> MTAPHDPLDDIQADPWALWLSGRT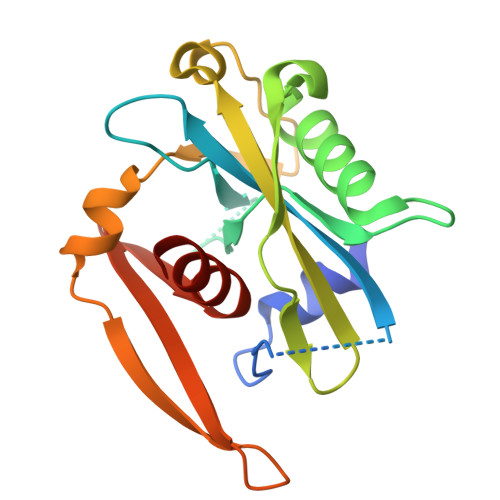RTALELPHYRRAAVLVALTREADPRVLLTVRSSELPTHKGQIAFPGGSLDAGETPTQAALREAQEEVALDPAAVTLLGELDDVFTPVGFHVTPVLGRIAPEALDTLRVTPEVAQIITPTLAELRAVPLVRERRTLPDGTEVPLYRYPWRGLDIWGMTARVLHDLLEQGPG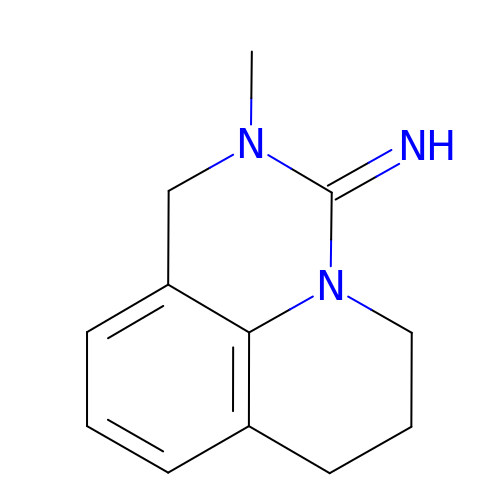2-methyl-1,2,6,7-tetrahydro-3H,5H-pyrido[3,2,1-ij]quinazolin-3-imine | C12 H15 N3 | STPBYFBWXRKLRN-OUKQBFOZSA-N Latrophilins, receptors for spider venom α-latrotoxin, are adhesion type G-protein-coupled receptors with emerging functions in synapse development. All LPHNs have a large ectodomain of approximately 1,000 amino acids, with an N-terminal lectin domain, followed by an olfactomedin-like (Olf) domain, a serine/threonine-rich region, HormR domain, and a GPCR-autoproteolysis inducing (GAIN) domain containing a GPCR proteolysis site (GPS). The N-terminal region binds the endogenous cell adhesion molecule FLRT, a major regulator of cortical and synapse development. Here we present the crystal structure of an N-terminal fragment of murine LPHN3 comprising the lectin and Olf domains (hereafter LPHN3Lec-Olf).

We expressed secreted murine LPHN3Lec-Olf in human embryonic kidney (HEK) 293T cells using established protocols to circumvent the formation of heterogeneous glycans (Aricescu et al., 2006), and determined the crystal structure to a resolution of 2.16 Å. The structure reveals two globular domains separated by a 17-residue linker (residues V192–K208). The structure of the LPHN3 lectin domain agrees closely with the lectin domain of LPHN1 solved using solution NMR (Vakonakis et al., 2008) (root-mean-square deviation [rmsd] is 0.86 Å for 90 aligned Cα atoms). The Olf domain folds into a five-bladed β propeller, with each blade consisting of a four-stranded β sheet. The fourth strands from blades I–IV largely form the periphery of the disk together with the Olf domain N terminus (β0), which contributes as the fourth strand to blade V. A disulfide bridge (C203–C385) connects the region upstream of β0 with blade IV and appears to stabilize β0 in its position. Notably for an extracellular protein, LPHN3Lec-Olf contains a reduced cysteine (C227) buried in the core of the Olf domain. In the electron density map, two potential metal atoms were visible approximately halfway through the central Olf channel. The result of this analysis points to calcium (CBVS = 1.767) and sodium (CBVS = 1.560) for the octahedrally coordinated and pentacoordinated ion, respectively. LPHN3Lec-Olf exhibits a sequence-conserved patch on the Olf domain, stretching across blades II and III of the propeller. We conclude that the FLRT-binding site involves conserved surface regions on blades II and III of the LPHN3 Olf domain.

> ETGPIPMAVVRRELSCESYPIELRCPGTDVIMIESANYGRTDDKICDSDPAQMENIRCYLPDAYKIMSQRCNNRTQCAVVAGPDVFPDPCPGTYKYLEVQYECVPYKVEQKVFLCPGLLKGVYQSEHLFESDHQSGAWCKDPLQASDKIYYMPWTPYRTDTLTEYSSKDDFIAGRPTTTYKLPHRVDGTGFVVYDGALFFNKERTRNIVKFDLRTRIKSGEAIIANANYHDTSPYRWGGKSDIDLAVDENGLWVIYATEQNNGKIVISQLNPYTLRIEGTWDTAYDKRSASNAFMICGILYVVKSVYEDDDNEATGNKIDYIYNTDQSKDSLVDVPFPNSYQYIAAVDYNPRDNLLYVWNNYHVVKYSLDFGPLDGTKHHHHHH>MDNKTYEISSAEWEVMNIIWMKKYASANNIIEEIQMQKDWSPKTIRTLITRLYKKGFIDRKKDNKIFQYYSLVEESDIKYKTSKNFINKVYKGGFNSLVLNFVEKEELSQDE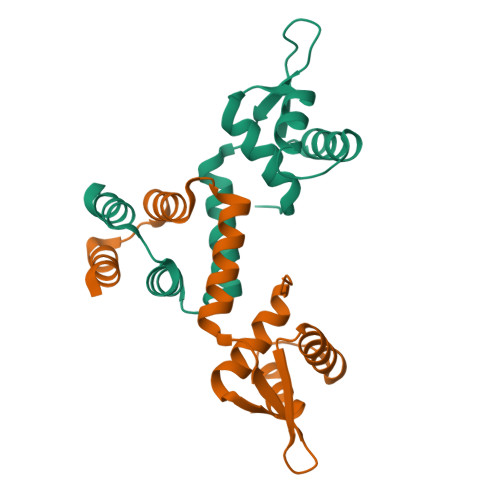IEELRNILNKK[2x]>[3x]AHAPGTDQMFYVGTMDGWYLDTKLNSVAIGAHWSCFIVLTITTFYLGYESWTSRGPSKRTSFYAGYQEEQNLALFVNFFAMLSYFGKIVADTLGHNFGDVGPFIIGFGNYRYADYMLTCPMLVYDLLYQLRAPYRVSCSAIIFAILMSGVLAEFYAEGDPRLRNGAYAWYGFGCFWFIFAYSIVMSIVAKQYSRLAQLAQDTGAEHSLHVLKFAVFTFSMLWILFPLVWAICPRGFGWIDDNWTEVAHCVCDIVAKSCYGFALARFRKTYDEELFRLLEQLGHDEDEFQKLELDMRLSSNGERLRRLSLNSLEVLFQ

ChRmine is a bacteriorhodopsin-like cation channelrhodopsin (BCCR) more closely related to ion pump rhodopsins than other channelrhodopsins. ChRmine displays unique properties favorable for optogenetics including high light sensitivity, a broad, red-shifted activation spectrum, cation selectivity, and large photocurrents, while its slow closing kinetics impedes some applications. ChRmine is a homotrimer with a central pore between subunits, unlike all other channelrhodopsins of known structure which are homodimers. The general topology of each ChRmine subunit is typical of rhodopsins, with an extracellular N-terminal region (amino acids 2–26), seven transmembrane helices (TM1-7, amino acids 27–270), intracellular and extracellular linkers (ICL1-3 and ECL1-3), a cytoplasmic C-terminal region.

To date, there are no channelrhodopsin structures without bound retinal and the structural consequences of retinal binding, which could have implications for the design of functional variants, are unknown. We purified apo-ChRmine from cells grown without addition of all-trans retinal, reconstituted it into lipid nanodiscs, and determined its structure to 4.1 Å resolution. The lower resolution of the apo structure is due in part to fewer particles and anisotropy of the reconstruction due to preferred particle orientation and potentially an increase in overall ChRmine flexibility. The apo-ChRmine structure (consisting of residues 3–285) was modeled by combining portions de novo built (into well-defined regions) with docked portions of the ATR-bound structure (into less well-defined regions) prior to structure refinement. The structures are similar overall (r.m.s.d. = 0.8 Å); no major rearrangements in the overall fold are observed. However, subtle conformational changes are focused to the intracellular halves of TM1, TM5, TM6, and TM7, which bow out toward the membrane ~0.5 Å, 1 Å, 2 Å, and 1 Å, respectively. The overall effect is to expand the retinal binding pocket and loosen packing between TM6 and its neighboring helices TM5 and TM7 on the membrane facing sides. These changes may facilitate loading apo-ChRmine with retinal.>[2x]YLEAFPKELREYYKNLFGKEEANKIMKKLREPVEHYYIRVNTLKISREKLIGELKKEGLKPLRSPYLPEGLYFVREGPNFSDDFEPKLPVVVANKYAAESVYQGAMLYAPGVLKADKNIKEGDEVQIRDPKGLLVGIGIARMDYKEMTEATRGLAVEVTLPKFKLPSLSELKAFEKGYFYPQGLPSMVTARVLEPKEDDVIIDMAAA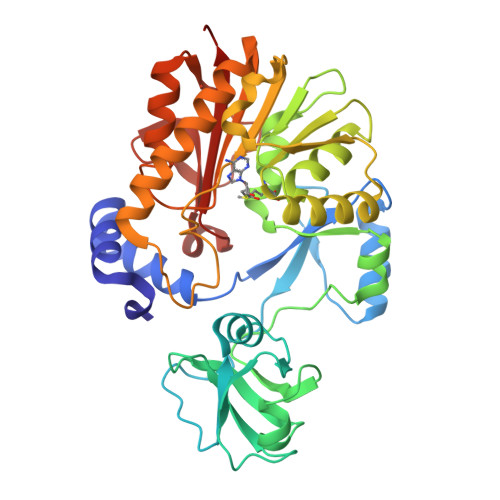PGGKTTHIAQLLENKGEIIAIDKSKNRLRKMEENIKRLGVKNVKLVQMDARKLPDLGIKADKILLDAPCTALGVRPKLWEERTLKHIEATARYQRAFIWAAIKSLRRGGVLVYSTCTLSYEENEGNVKFMIRKGMKLEEQSIFIGSPGIGMNKVQRFYPHKHLTQGFFIAKLRKVKD> GSHMASSDDVTVVYQNGLPVISVRLPSRRERCQFTLKPISDSVGVFLRQLQEEDRGIDRVAIYSPDGVRVAASTGIDLLLLDDFKLVIND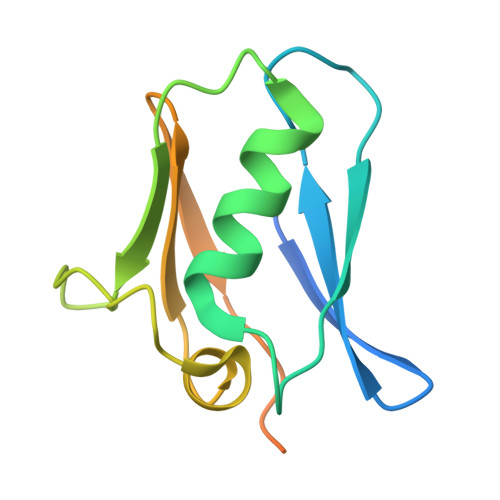LTYHVRPPKRDLLSHENAATLNDVKTLVQQLYTT>MASTYKVHYFDFTGRAEPIRMILSYGKLDFEDVRVSREEFQKLKPTLPLGQLPVLEFQGHMIPQSTAICRFLANKANLSGKDEFENLKIDVAVDTIEDLKKKVSEWAYEKNEEKKKALEETTLKEHVPFFLKKLEIHAEKNGGYLALNRISWADIIFLCAYETLGNMLKKDILIDYPNLTKVKQNILEVPSIKEWIKKRPTNPMLS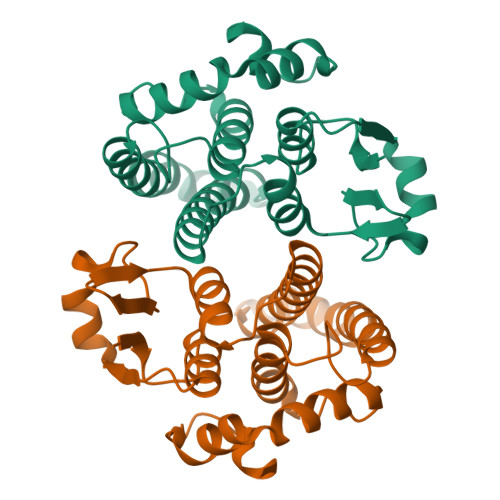FDLKSQVLEHHHHHH[4x]Although no X-ray crystal structure of human GBA2 is available, structures have been solved for Thermoanaerobacterium xylanolyticumTxGH116 β-glucosidase, which shares 37% amino acid sequence identity with human GBA2.8 Instead of hydrolyzing glucosylceramide like GBA2, TxGH116 exhibits high activity toward 4-nitrophenyl β-D-glucopyranoside (4NPGlc), and β-1,3- and β-1,4-linked glucooligosaccharides. The TxGH116 structure contains an N-terminal domain, formed by a two-sheet β-sandwich, tightly associated with a C-terminal (α/α)6 solenoid domain that contains the catalytic nucleophile, E441, and general acid/base, D593, residues, which were verified by chemical rescue of alanine mutants. GH116 enzymes are retaining GHs, as shown for Saccharolobus solfataricus SSO1353 β-glucosidase/β-xylosidase, human GBA2, and TxGH116.6,8,12 In the retaining mechanism, catalysis involves two carboxylic acid/carboxylate side chains with one serving as an acid/base and the other as a nucleophile. Here, we report the structures of Thermoanaerobacterium xylanolyticum β-glucosidase (TxGH116) D593N acid/base mutant in complexes with cellobiose and laminaribiose and its catalytic mechanism.

Indeed, the activities of the D593E, D593G, and D593N mutants were reduced by 36-, 3300-, and 140-fold relative to wild-type for hydrolysis of 4NPGlc, respectively, and in the ranges of 250–900-, 20 000–36 000- and 39 000–44 000-fold for hydrolysis of oligosaccharides. The decreased activities were verified by kinetic analysis of D593A and D593N, which showed ∼30 000-fold decreases in the apparent kcat/Km values relative to wild-type. These data support the action of D593 as the catalytic acid in the reaction mechanism and indicate the mutants are slow enough catalysts to soak with substrates to obtain Michaelis-complex-like structures. In all structures, the acid/base residue was mutated to asparagine (D593N) or alanine (D593A). The D593A and D593N unliganded enzymes and D593N complexes crystallized in the space group P21212, isomorphous, with wild-type TxGH116 crystals, whereas the crystals of TxGH116 D593A in complex with cellobiose and laminaribiose crystallized in the P212121 space group and had 2 molecules in one asymmetric unit. The overall structures of unliganded TxGH116 D593A and D593N, and in particular the position of amino acid residues in the active sites, were similar. However, the loops of residues 523–534 and 583–597, the last containing the mutated acid/base residue, as well as the side chains of D452 and Q727 in the active site differed from those of wild-type TxGH116. The distance between the catalytic nucleophile E441 and mutated catalytic acid/base N593 in TxGH116 D593N (10.6 Å) was longer than the distance between E441 and the catalytic acid/base D593 in the wild-type TxGH116 structure (8.5 Å).

> AMALTGCSEKININEDKISHKIDIPDSAWTIGIGEKFKNAGHPNVKYPMIDDSYVQGAPLGGFGAGTIGRTYNGGFSRWHLEIGKNKYTTVYANQFSVFQKVEGNKDGVAQVLYAGEPENGYLSSWKWDYPKESGMYYALYPNSWYTYTNKDLPVQLAVKQFSPIIPYNYKETSYPVAVFKWTAYNPTNKNVDVSIMFTWQNMIGFFGKQVNVNSGNFNKIIKDKSKDSEIVAAVMGNISNDNEEWNGEYSIGVKKVPGVDISYKAKFVTTGDGSDLWHEFSKNGILDNKDDETPTKQDGIGSAIAVNFKLQPGQTIEVPFALSWDLPIMKFGGGDKWYKMYTKYFGKNGKNSFAILKEALNNYQKWEKMIDDWQKPILSNKSKPDWYKTALFNELYYLADGGTAWENGKVGEKDKRTNNMFGLLECFDYNYYETLDVRFYGSFPLVMLWPDIEKQVMRQFADTINVQDSSEFKVGSNGAMAVKKVQGMIPHDLGSSYALPWIKINAYDWQNPNIWKDLNSKYVLLVYRDYVLTGKTDKEFLKYTWKSVKTALDKLKEMDKDNDGIPDNEGIPDQTYNTWSMKGTSAYCGSLWLAALKAAQEIGKVLKDNEAYIKYNEWYKIAQQNFEKELWNGEYYNFDTESDHKDSIMADQLAGQWYADILRLGDILPKDHVQKALKKIYEFNVMKFENGKMGAVNGMRPDGIVDESDIQAQEVWTGVTYALASFMKYRGMTEEAYNTAYGVYKMTYDKSGKGYWFRTPEAWTKDGNYRASMYMRPLSIWSMEVNYNEVLEHHHHHH>[2x]SKPFTVPILTVEEMSNSRFPIPLEKLYTGPSSAFVVQPQNGRCTTDGVLLGTTQLSAVNICNFRGDVTRVGISHDYTMNLVSQNWNNYDPTEEIPAPLGTPDFVGKIQGLLTQTTRADG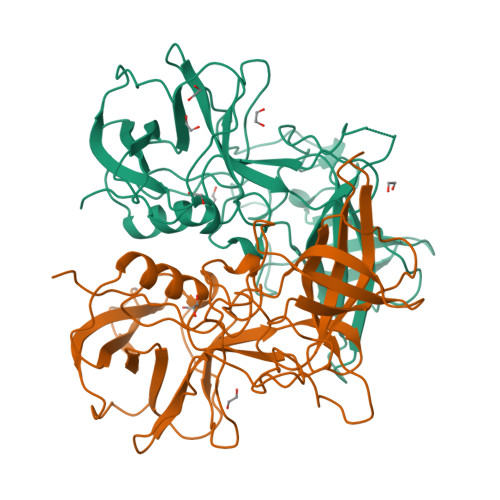STRAHKATVSTGSVHFTPKLGSVQFTTDTNNDFQTGQNTKFTPVGVIQDGDHHQNEPQQWVLPNYSGTSGHNVHLAPAVAPTFPGEQLLFFRSTMPGCSGYPNMNLDCLLPQEWVSHFYQEAAPAQSDVALLRFVNPDTGRVLFECKLHKSGYITVAHTGPYDLVIPPNGYFRFDSWVNQFYTLAPM> GAMEPLIDPYTQTNAVSYERFIRWYSKENHISATTEDLYNSLHGTYN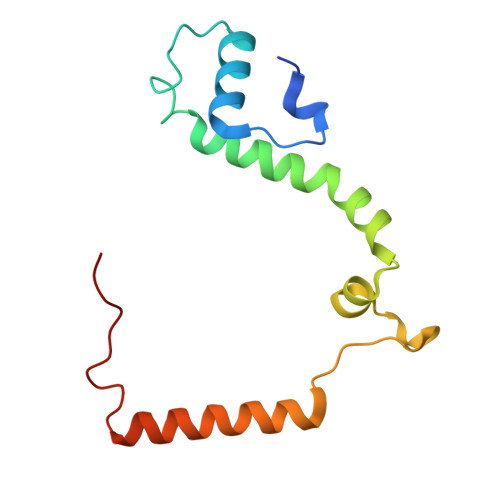NYKQDLYARTARSFVESHCDEAWFEDSYWVDESQGRVLEVSENEKSYRRALYDKFMDRLDAGYYDDFQLPTAE> GPLGSMWERLNCAAEDFYSRLLQKFNEEKKGIRKDPFLYEADVQVQLISKGQPNPLKNILNENDIVFIVEKVPLEKEETSHIEELQSEETAISDFSTGENVGPLALPVGKARQLIGLYTMAHNPNMTHLKINLPVTALPPLWVRCDSSDPEGTCWLGAELITTNNSITGIVLYVVSCKADKNYSVNLENLKNLHKKRHHLSTVTSKGFAQYELFKSSALDDTITASQTAIALDISWSPVDEILQIPPLSSTATLNIKVESGEPRGPLNHLYRELKFLL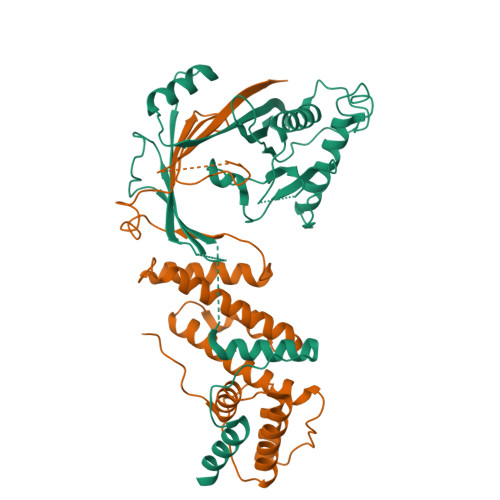VLADGLRTGVTEWLEPLEAKSAVELVQEFLNDLNKLDGFGDSTKKDTEVETLKHDTAAVDR;> SVKRLFKVRSDLDFAEQLWCKMSSSVISYQDLVKCFTLIIQSLQRGDIQPWLHSGSNSLLSKLIHQSYHGTMDTVSLSGTIPVQMLLEIGLDKLKKDYISFFIGQELASLNHLEYFIAPSVDIQEQVYRVQKLHHILEILVSCMPFIKSQHELLFSLTQICIKYYKQNPLDEQHIFQLPVRPTAVKNLYQSEKPQKWRVEIYSGQKKIKTVWQLSDSSPIDHLNFHKPDFSELTLNGSLEERIFFTNMVTCSQVHFK>[2x]GMILSAEQSFTLRHPHGQAAALAFVREPAAALAGVRFLRGLDSDGEQVWGELLVTVPLLGEVDLPFRSEIVRTPQGAELRPLTLTGERAW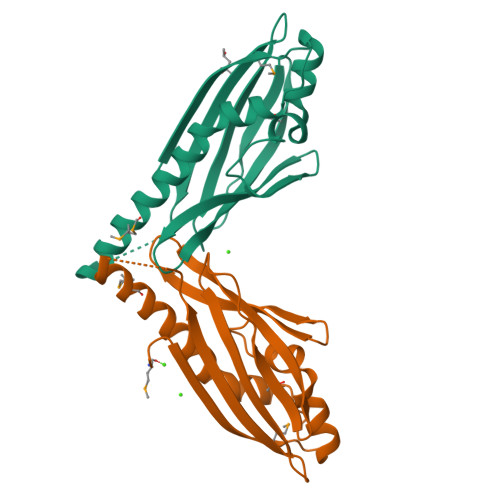VAVSGQATAAEGGEMAFAFQFQAHLATPEAEGWGGAAFEKMVQAAAGRTLERVAKALPEGLAAGLPPA> QINQV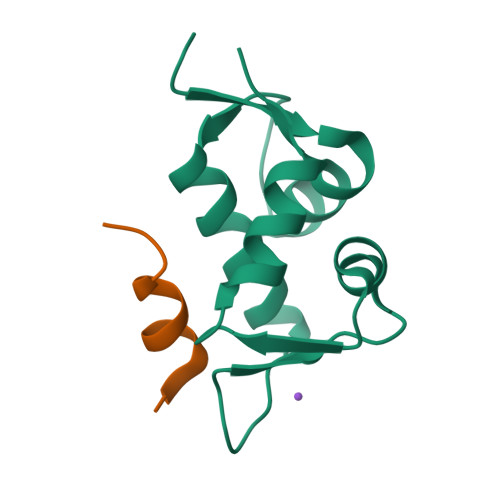RPKLPLLKILHAAGAQGEMFTVKEVMHYLGQYIMVKQLYDQQEQHMVYCGGDLLGELLGRQSFSVKDPSPLYDMLRKNLVTLAT;> LTFEHYWAQLTS β-lactamases inactivate β-lactam antibiotics by hydrolyzing and “opening” their signature β-lactam ring. In serine-based β-lactamases of Class A, C and D, this hydrolytic process is executed in the deacylation step involving an activated water molecule carrying out nucleophilic attack on the enzyme-substrate acyl adduct ES*. Here we report structural and computational studies of Class A β-lactamase PenP with Glu166Tyr mutation that analyze the interactions between this critical water molecule, termed WAT_Nu, and other components of the active site during a full cycle of hydrolysis. In summary, by analyzing the reaction intermediates observed in the active site of a Class A β-lactamase hydrolyzing a β-lactam substrate, our study has uncovered critical features within the active site that coordinate and activate the water molecule for hydrolysis.

In the active site of the apo structure, the mutated residue Tyr166 adopts the same conformation as the Glu166 residue in the wild-type structure but the bulky side chain of Tyr166 extends much closer toward the catalytic residue Ser70 and forms a stable hydrogen bond with it (distance ~2.8 Å). The Glu166Tyr mutation has little impact on the overall structure of the active site as nearby residues like Ser70, Lys73 and Asn170 adopt essentially identical conformation as in wild-type structure. Notably, the key catalytic water molecule, termed WAT_Nu for its potential role as the hydrolytic nucleophile, forms totally six hydrogen bonds with partners including the side chains of Ser70, Tyr166 and Asn170 as well as the mainchain carbonyl of Ala237, the main chain amide of Ser70 plus a possible sulfate ion from the bulk solvent. Compared to a similar water molecule observed in the wild-type TEM-1 structure, WAT_Nu in Glu166Tyr mutant structure is located closer to Ser70 and Asn170, but farther away from Lys73. This difference is probably due to the bulkier side of Tyr166 as compared to Glu166, resulting in WAT_Nu being “pushed” away from Lys73 and toward Ser70 instead. In the apo structure with ES* absent, WAT_Nu is coordinated by a network of hydrogen bonds involving Glu166Tyr, Asn170 and Ala237.

>GPMKTEMKDDFAKLEEQFDAKLGIFALDTGTNRTVAYRPDERFAFASTIKALTVGVLLQQKSIEDLNQRITYTRDDLVNYNPITEKHVDTGMTLKELADASLRYSDNAAQNLILKQIGGPESLKKELRKIGDEVTNPERFYPELNEVNPGETQDTSTARALVTSLRAFALEDKLPSEKRELLIDWMKRNTTGDALIRAGVPDGWEVADKTGAASYGTRNDIAIIWPPKGDPVVLAVLSSRDKKDAKYDDKLIAEATKVVMKALNMNGK[2x]>[2x]MSRQASRLDAKKVNSEFLTLTYGALVTQMLRDFENAEDVNKQLERIGYNMGMRLIEDFLARTSAPRCLEMRETADRIQQAFRIYLNIQPTISNWSPASDEFSLVFDSNPLTEFVELPPDLTNLRYSAILSGCIRGALEMVQLEVQCWFVQDQLKGDNVTELRVKFVRRLEEVIPAGED;> MSEEILFDCLHAEIVNYCLDSNKEHDLATLEYIGFTTGYRLIERLTREVSRFKDELETMKFICTDFWMLIYKKQVDNLRTNNHGMYVVQDKAFRFLTRISPGTKQLEHAPKFVAFTCGLVRGALSNLGINSTVTAEVQSIPACKFHIEVNRN;> MTIFNLYIFDKFGTLLHYAEWNRTKKSGITREEEAKLTYGMLFSIKSFVSKISPHDPKEGFLYYKTNRYALHYLETPSGLKFVLNTDTTAINVKELLQQLYAKVWVEFVVRDPLWTPGTVVTSELFQSKLDEFVRQSPIFGIRNI;> MIIYGVYIVSKSGGLIFNLDNNVPRIEHEKTFTYPLDLVLDYDSKKVSVSFNRKDGINVGHVLVAVNGMPVNGVTLDDGRDVRTTLDAPENYPINLKFSRPKMTTNEKIFLASMFYPLFAIASQLSPEPKSSGIEILEADTFTLHCFQTLTGIKFIIISETGLNGIDLLLRKVYELYSDYVLKNPFYSLEMPIRCELFDNKLQELLAQVEKTGISNIDK;> MSTYYFVIVGQNDNPIYEKEFSTVNKELRKEDHRHLTQFIAHAALDLVDEHKWKTANMQLKSIDRFNQWFVSAFITASQIRFIIVHDNKNDEGIKNFFNEMYDTYIKNSMNAFYRINTPIKSPMFEKKSEIFGRKYLLS;> MEKLEALKISSMRPRSNILDRPLSKGKTEVSQSIVALLFSEIVQYSQSRVFTVPELQTRLHDLGQDVGTRIIDLYFVRERSSKRETKLTQMLLFVKTTVWKNLFGKEAEKLEHANDDERTYYIIEKEPLVNTFISVPKDKGSLNCANFTAGIVEAVLTNCGFPCKVTAHWHKGTTYMVKFEDFVIARDKQMEEK;> MAFCIAVIGKDNAPLYLTTSDMEQELELQYHVNAALDVVEEKCLIGKGAPESKELYLGLLYSTENHKIYGFVTNTRVKFIVVIDSSNVALRENEVRAIFRNLHLLYTDAICNPFYIPGESLTSKKFDRAVQKLMSGTA;> DNLRHFVQDYAVRALIPYIEHLVAILAEGVTNKKGVSKSLLSATKRWFVTSKPGAGANNQNAVIYTNESAELQTRKLGDLYFMFGHYNLAFQSYHQAKRDFNADSAWQYYAGALEMAALSAFMLGTAQRKTYDYMEDAIVCYLTVCKLQQFATRATLLSMECLKTARLYSEVAKQLIRMTNEESDLRSALLLEQAAYCFLVTQPPMHRKYAFHIVLAGNRYSRAGQRKHAYRCYRQAYQVFQKREW;> MTMDATALPSELLVTPQPLVGFCGLDTARVSVHKAVWEAFSGSLQRKAADRAAVQYKLLPPNYEFPVAKPKRASYEWYHPKGILKRNWMLKHLHVLPSVVVLFQDMEWNDLQWTEKQVQCAAIVQALKNTLQERNTRLCLVLLQRAAPLPPGEDLLAAERAASLTNACGITSKMLFILPHTEHLTGYALRLESAFLDMAQSYYALMSKRIRNHRDQLTAAHTSLKIRHQFKLGFVAEMRQDFSTGQKHYFQAYANLDEIRINDGNCLEIKTLAGFLNYKICRLMFKLKTPRDAINQFIIHVEKHKSRVGFKDLAFEHHAWLSTQHSVFAELFCEAIKNGLPALQTQHPGIYYHKAAEFVMKRRDAAMEAYAAMQASSEATPTPIQNPLSLYTEFFGIRAVKTGDLVAEQQANMQLCDQERSYNHSAAIIALLSQAMAQFKIYKCLRFRKKLAIDMAEEYLKSGDHAKALTLYSLMLPDYRQEKWTTIFTDVLLKTLRCALLSGSVADYIACSVEALSLRHQSDQSERILILENLWQVFQGVPPMPKTQLTPEAQALWTSALANVKSPIQIDLDKVNDVVEMCATFERVQLSNDDLLQLQLIVRVLTDIPLRIRSFHVILADAGNPQNSYKLEALKYFCFPTLTQLRGQKQPDDEQLENPSQEPKNFEKNMRLEPGSYYQLFCSTEAQQFHENTQLRIVRLEAHMGTDQVAALLTCSSN

The TRAPP complexes are nucleotide exchange factors that play essential roles in membrane traffic and autophagy. TRAPPII activates Rab11, and TRAPPIII activates Rab1, with the two complexes sharing a core of small subunits that affect nucleotide exchange but being distinguished by specific large subunits that are essential for activity in vivo. We report a cryo‐EM structure of the entire Drosophila TRAPPIII complex. The TRAPPIII‐specific subunits TRAPPC8 and TRAPPC11 hold the catalytic core like a pair of tongs, with TRAPPC12 and TRAPPC13 positioned at the joint between them.

Expressing TRAPPIII without the TRAPPC12 and TRAPPC13 subunits reduces its size by ~100 kDa, close to the combined weight of two subunits, indicating that their absence does not affect the binding of the other nine subunits (Fig EV1, EV2, EV3, EV4). This “miniTRAPPIII” complex is still able to activate Rab1 but, like the complete complex, it has no detectable activity on Rab11 (Fig EV1E). Moreover, in the case of the miniTRAPPIII, similar narrow rod and triangular particles were found in the cryo‐EM micrographs, but threefold symmetrical particles rarely appeared among the 2D class averages. We reanalysed cryo‐EM images of miniTRAPPIII following a similar strategy to that used for TRAPPIII. The comparison between the TRAPPIII and miniTRAPPIII class 2D averages and 3D models revealed that the flat rod was similar, but in miniTRAPPIII there was density missing at the region of interaction between the two arms. We concluded TRAPPC12 and TRAPPC13 were located in this region of TRAPPIII, forming one of the vertexes of the triangle.> SLWQFGKMINYVMGESGVLQYLSYGCYCGLGGQGQPTDATDRCCFV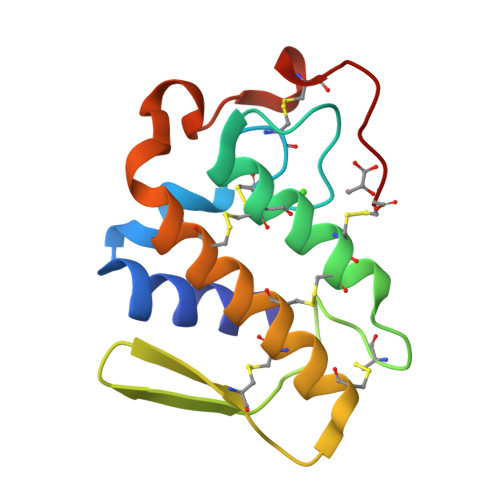HDCCYGKVTGCNPKIDSYTYSKKNGDVVCGGDNPCKKQICECDRVATTCFRDNKDTYDIKYWFYGAKNCQEKSEPC>GPGSELPQMVQQLNSPDQQELQSALRKLSQIASGGNEQIQKLIEAGALSPLVKLLDDASEEVIKEAVWAIANIASGNNEQIQKLIEAGALSPLVKLLDDASEEVIKEAVWAIANIASGNNEQIQKLIEAGALSPLVKLLDDASEEVIKEAVWAIANIASGNNEQIQKLIEAGALSPLVKLLDDASEEVIKEAVWAIANIASGNNEMKQKLEEAGALPALEKLQSHANEEVQKNAQAALEAFNS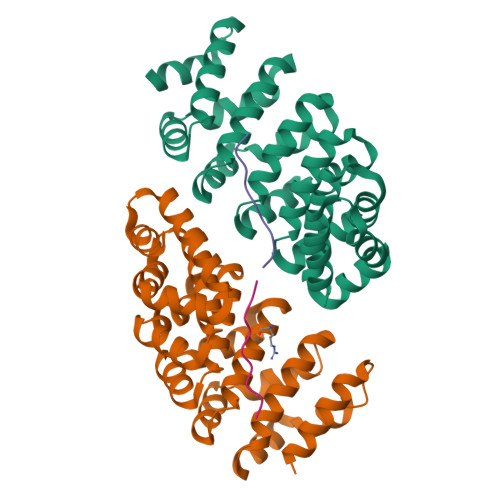[4x];>[4x]RRRRRRRRRR> AELTPEVLTVPLNSEGKTIT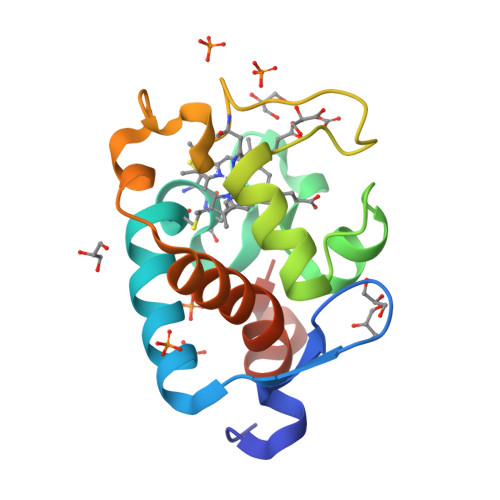LTEKQYLEGKRLFQYACASCHVGGITKTNPSLDLRTETLALATPPRDNIEGLVDYMKNPTTYDGEQEIAEVHPSLRSADIFPKMRNLTEKDLVAIAGHILVEPKILGDKWGGGKVYY>MAGYGAKGIRKVGAFRSGLEDKVSKQLESKGIKFEYEEWKVPYVIPASNHTYTPDFLLPNGIFVETAGLWESDDRKKHLLIREQHPELDIRIVFSSSRTKLYKGSPTSYGEFCEKHGIKFADKLIPAEWIKEPKKEVPFDRLKRKGGKK[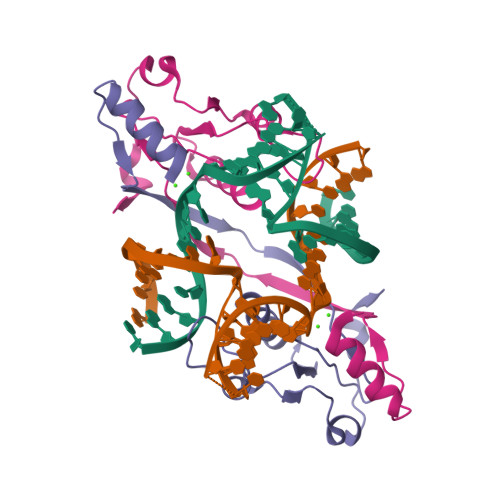2x]> CSNASVLDPKGPVAEQQSDLILLSIGFMLFIVGVVFVLFTIILVKYRDRKGKDNGSYNPEIHGNTFLEVVWTVIPILIVIALSVPTVQTIYSLEKAPEATKDKEPLVVYATSVDWKWVFSYPEQDIETVNYLNIPVDRPILFKISSADSMA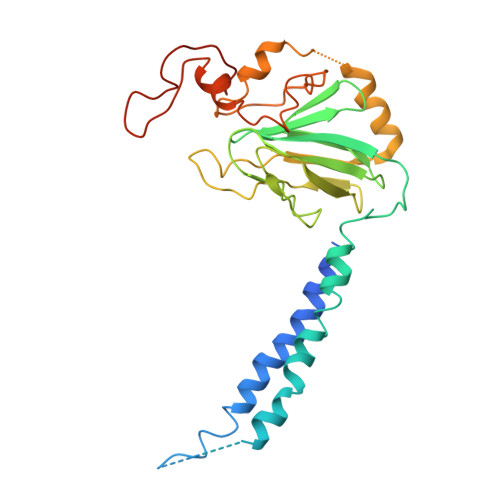SLWIPQLGGQKYAMAGMLMDQYLQADKVGTYEGRNANFTGEHFADQEFDVNAVTEKDFNSWVKKTQNEAPKLTKEKYDELMLPENVDELTFSSTHLKYVDHGQDAEYAMEARKRLGYQAVSPHSKTDPFENVKKNEFKKSDDTEE>[4x]M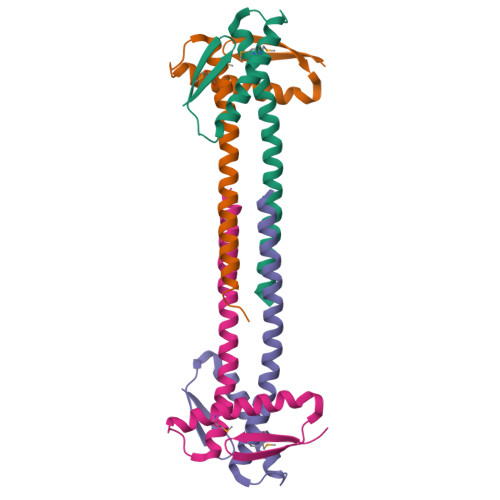SQSNTLTVQILDKEYCINCPDDERANLESAARYLDGKMREIRSSGKVIGADRVAVMAALNITHDLLHRKERLDQESSSTRERVRELLDRVDRALANPADAGEA S-(3-methylbut-2-en-1-yl) trihydrogen thiodiphosphate | C5 H12 O6 P2 S | 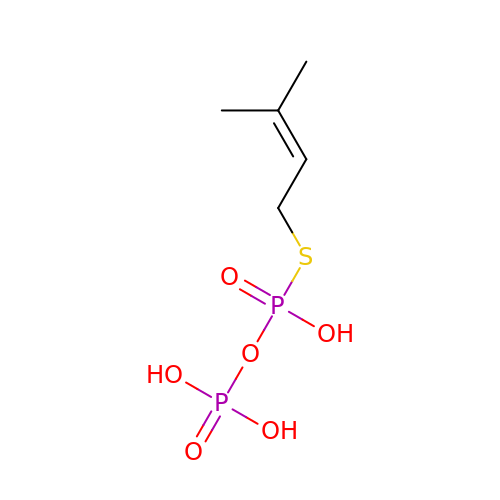ZWFWSISPSBLNGO-UHFFFAOYSA-N> QS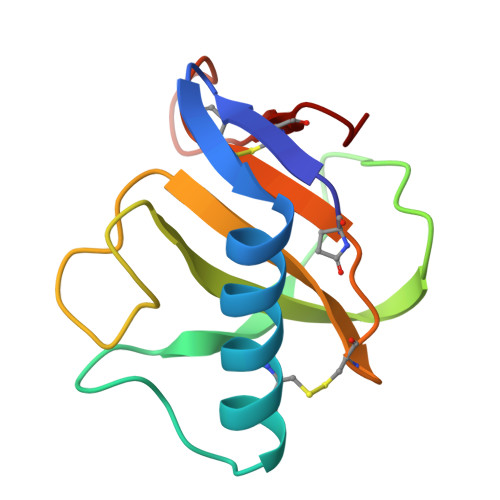ATTCGSTNYSASQVRAAANAACQYYQNDDTAGSSTYPHTYNNYEGFDFPVDGPYQEFPIKSGGVYTGGSPGADRVVINTNCEYAGAITHTGASGNNFVGCSGTN>MKILFVASGSPATVFALAPLATAARNAGHDVFMGAVEDMVPYIASAGIPALSIAPSSIRRYATMDREGNPVRMPETPEEELDFAGHWFGRMAAGS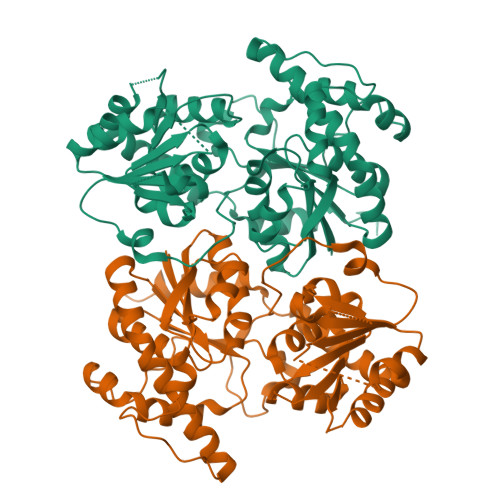MDALREVTANWRPDLVVGGSMSFAAALIAAELGVPYVRQAWDTGDAWRTDPAASDELRPELRALGLDRLPDPALFVDICPPSLRPATAPPAQMMRWVPANGQRRLEPWMYTKGNRPRILVTSGSRLVFAKKTGFLRGLVADMAALDAEVVIATLDEVAEELRTELPGVRAGWVPLDVVVPTCDVVVHHAGGVTALTAMNAGVPQLIVPQGGNFVEAGLRISDFGAAITVDENTPEAVEKACGELIGNPSYAERARELSAEIAALPLPAEVVGALEGLVENLYFQ[2x]> KETAAAKFERQHMDSSTSAASSSNYCNQMMKSRNLTKDRCKPVNTFVHESLADVQAVCSQKNVACKNGQTNCYQSYSTMSITDCRETGSSKYPNCAYKTTQANKHIIVACEGNPYVPVHFDASVGPPGKETAAAKFERQHM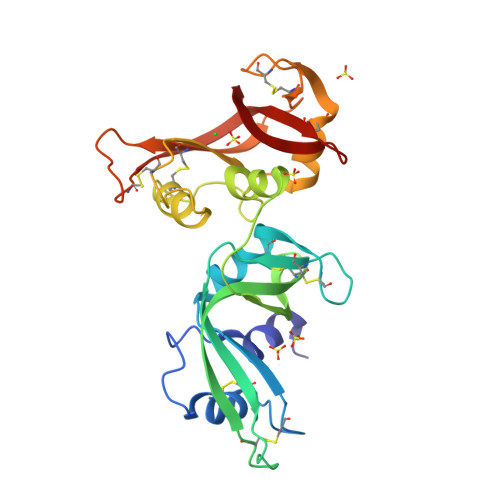DSSTSAASSSNYCNQMMKSRNLTKDRCKPVNTFVHESLADVQAVCSQKNVACKNGQTNCYQSYSTMSITDCRETGSSKYPNCAYKTTQANKHIIVACEGNPYVPVHFDASV> MAHHHHHHVDDDDKIRDISSKELIKEMNFGWNLGNTMDAQCIEYLNYEKDQTASETCWGNPKTTEDMFKVLIDNQFNVFRIPTTWSGHFGEAPDYKIDEKWL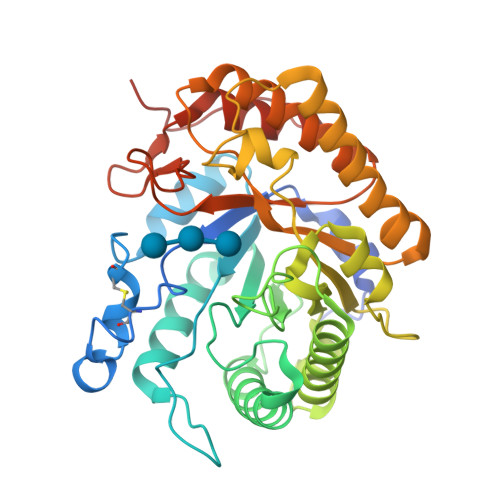KRVHEVVDYPYKNGAFVILNLHHETWNHAFSETLDTAKEILEKIWSQIAEEFKDYDEHLIFEGLNAPRKNDTPVEWTGGDQEGWDAVNAMNAVFLKTVRSAGGNNPKRHLMIPPYAAACNENSFNNFIFPEDDDKVIASVHAYAPYNFALNNGEGAVDKFDAAGKRDLEWNINLMKKRFVDQGIPMILGEYGAMNRDNEEDRATWAEFYMEKVTAMGVPQIWWDNGVFEGTGERFGLLDRKNLKIVYPTIVAALQKGRGLEVNVVHAIEKETEE> PSCVMDDFRDPQRWKECAKQGKMPCYFDLIEENVYLTERAKNKSHRDIKRMQCECTPLSKDERAQGEIACGEDCLNRLLMIECS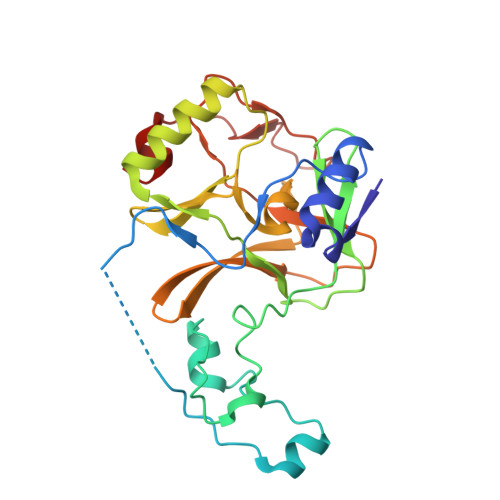SRCPNGDYCSNRRFQRKQHADVEVILTEKKGWGLRAAKDLPSNTFVLEYCGEVLDHKEFKARVKEYARNKNIHYYFMALKNDEIIDATQKGNCSRFMNHSCEPNCETQKWTVNGQLRVGFFTTKLVPSGSELTFDYQFQRYGKEAQKCFCGSANCRGYLGGENRVSIRAAGGK> STGSATTTPIDSLDDAYITPVQIGTPAQTLNLDFDTGSSDLWVFSSETTASEVDGQTIYTPSKSTTAKLLSGATWSISYGDGSSSSGDVYTDTVSVGGLTVTGQAVESAKKVSSSFTEDSTIDGLLGLAFSTLNTVSPTQQKTFFDNAKASLDSPVF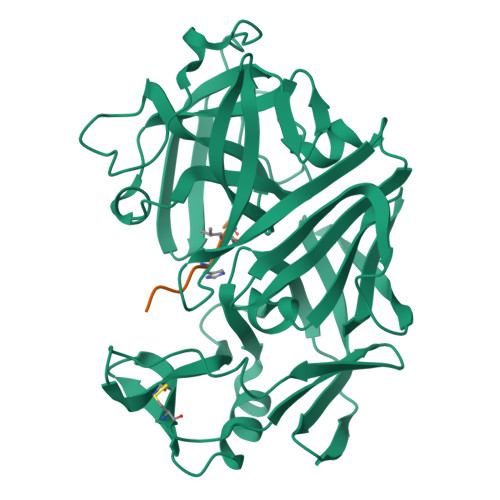TADLGYHAPGTYNFGFIDTTAYTGSITYTAVSTKQGFWEWTSTGYAVGSGTFKSTSIDGIADTGTTLLYLPATVVSAYWAQVSGAKSSSSVGGYVFPCSATLPSFTFGVGSARIVIPGDYIDFGPISTGSSSCFGGIQSSAGIGINIFGDVALKAAFVVFNGATTPTLGFASK;> PHPFHXVIHK>[2x]GAMGDFSFIKALQTAQQNFVVTDPSLPDNPIVYASQGFLNLTGYSLDQILGR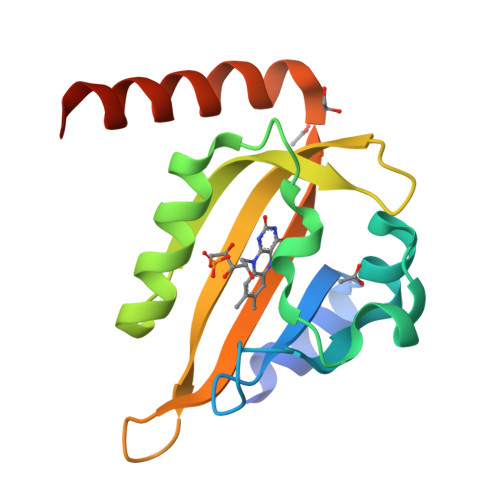NCRFLQGPETDPKAVERIRKAIEQGNDMSVCLLNYRVDGTTFWNQFFIAALRDAGGNVTNFVGVQCKVSDQYAATVTKQQEEEEEAAANDDED> MTESTLAFVFPGQGSQSLGMLAELSELHPQIRETFAEASEGAGVDLWALSQGGPEEMLNRTEYTQPALLAAGVAVWRLWTAQRGQRPALLAGHSLGEYTALVAAGVLSLHDGAHLVRLRGQFMQAAAPAGVGAMAAVLGAEDAVVLEVCAEAAGSQVVVPANFNSPGQIVIGGDAAAVDRALALLAERGVRKAVKLAVSVPSHTPLMRDAANQLGEAMAGLSWHAPQIPVVQNVDARVHDGSAAIRQALVEQLYLPVQWTGCV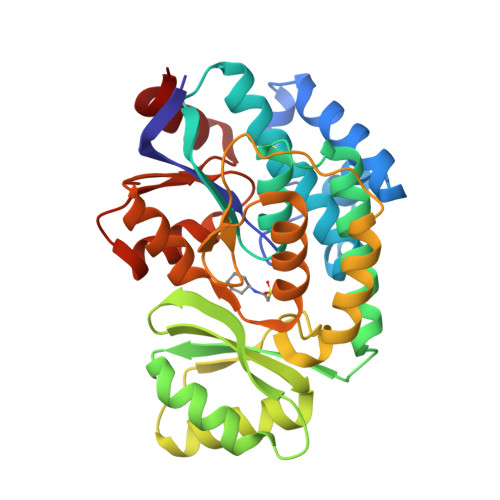QALASQGITRIAECGPGKVLSGLIKRIDKSLDARPLATPADYAGALDAWAH Here, we report the first structure of glycerol kinase from the thermophilic filamentous fungus Chaetomium thermophilum (CtGK). Glycerol kinase (EC 2.7.1.30) catalyzes the transfer of phosphate moiety from ATP to glycerol to form glycerol 3-phosphate (G3P). Overall, the CtGK polypeptide chain can be divided into two distinct domains classified by Pfam as FGGY_N (residues 65–325) and FGGY_C (residues 331–583) connected by a flexible region. A similar case is found in CtGK, which forms extended dimers via the interaction between the C-terminal domains with a prominent contribution from hydrophobic residues (Phe422, Gly436, Phe389, Leu394, Thr437, Phe439, Gly440, Ile441, Thr437, Thr445, Leu438, Ile450, Trp580).

We initially determined CtGK in an apo form using ethylene glycol as a cryoprotective agent. Initial molecular replacement efforts using a conventional approach were unsuccessful, we, therefore, decided to solve the structure using a MoRDa automated structure refined pipeline. The asymmetric unit (ASU) contained two polypeptide chains. The electron density map allowed for building the residue ranges 65 (or 67 for chain B) to 583. A short loop of 8 (or 9) amino acids (542–548/9) connecting the α-helix H18 and a β-strand S18 could not be modeled due to insufficient electron density. This likely reflects the high flexibility of this loop. The physiological dimer is not contained in the ASU but completed by a symmetry-related chain forming a rather elongated assembly (A:B’ and B:A’). The dimer interaction is mostly mediated by β-strands located on the C-terminal domains. Although crystals were grown from the same condition, the collected datasets were processed in different space groups. We observed that in the absence of nucleotide, CtGK adopts open conformation, which upon nucleotide binding closes up.

>GSFVGSIDQGTTSSRFLIFNGEGNPVASHQIEFENLYPKSGWHEQDPYELLNSVQQCIDGAMHKFASLGYSKENIRAIGITNQRETTVVWDSVTGEPLHNAIVWPDTRTSALVRELKARQSADSLLELCGLPLSTYPSSVKLLWLIQNVDAVKQAYEEGRLAFGTVDSWLIYKLNGGAQAERPIHVTDSTNASRTMFMNLRTLQYDDKLLGFFGIDRNKIKLPKIVPSSDPEAFGKVATGALAGVPIAGCLGDQSSALVGQCGFSPGQAKNTYGTGCFLLYNVGTEPVISKYGLLATVAYDFGRGRKPVYALEGSIAVAGAGITFLMNNLGFAPKPSEINALAESVLDNGGVVFVTAFSGLFAPYWIDDAKGTLFGITQHTTKGHIARATLEATCYQTRAILDAMEKDSGHKLESLAVDGGLSASDLCMQTQADISGIPVDRPRMRETTALGAAIAAGLATGVWRELDHVKESIAGGANGNGKKNAREVFYPKMDRKKAERLFRKWEQAVEMSRGWVREQEEEDGE[2x]>[7x]FDASNFKDFSSIASASSSWQNQSGSTMIIQVDSFGNVSGQYVNRAQGTGCQNSPYPLTGRVNGTFIAFSVGWNNSTENCNSATGWTGYAQVNGNNTEIVTSWNLAYEGGS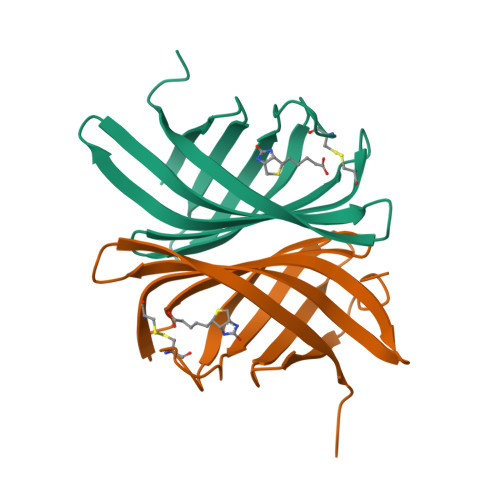GPAIEQGQDTFQYVPTTENKSLLKD Bacteriophage (phage) vB_EcoM_CBA120, discovered by Kutter and colleagues, is a member of the recently defined Kuttervirus genus of contractile tailed phages belonging to the Ackermannviridae family. Each TSP recognizes a different lipopolysaccharide on the membrane of a different bacterial host. The 335 N-terminal residues of TSP4 promote the assembly of the TSP complex and anchor it to the tail baseplate.

However, the SeMet TSP4-N335 containing three constitutive methionines and three additional engineered methionines designed to increase the anomalous signal (Leu12Met, Ile31Met and Leu145Met), were all twinned when grown in KNa-tartrate solution. Thus, phase determination was performed with SeMet protein crystals grown from solutions containing lithium sulfate. The diffraction quality was rather poor and required five merged data sets to yield sufficient anomalous diffraction signal for the identification of 15 Se sites, corresponding to 5 SeMet residues per monomer. Phase determination by the SAD method yielded an electron density map that enabled the building of the AD-XD1-XD2 trimer. However, the electron density associated with the XD3 domains could not be traced. The crystal structure of TSP4-N335 reveals a trimeric protein comprising four domains. The XD2 and XD3 domains share the same threefold symmetry axis as the AD and XD1 domains such that three XD2 domains splay apart and do not interact with one another whereas the three XD3 domains pack together around the threefold symmetry axis. A linker (Gly179-Leu-Gly-Gln-Gly-Arg-Val-Tyr-Ser-Arg188) that connects the XD1 and XD2 domains exhibits a well-defined conformation in the two TSP4-N335 crystal structures. The third linker connects the TSP4 XD2 and XD3 domains by a glycine-rich flexible long polypeptide (Thr250-Pro-Ile-Gln-Leu-Gly-Asn-Gly-Gly-Gly-Ser-Gly-Ser-Ser-Thr264) that is structurally disordered as manifested by the lack of associated interpretable electron density maps for both the wild-type and SeMet TSP4-N335 crystal structures.

>MANKPTQPLFPMGLETSESSNIKGFNNSGTMEHSPGAVMTFPEDTEVTGLPSSVRYNPDSDEFEGYYENGGWLSLGGGGIRWETLPHAPSSNLLEGRGYLINNTTGTSTVVLPSPTRIGDSVTICDAYGKFATYPLTVSPSGNNMYGSTEDMAITTDNVSATFTWSGPEQGWVITSGVGLGQGRVYSREIFTQILASETSAVTLNTPPTIVDVYADGKRLAESKYSLDGNVITFSPSLPASTELQVIEYTPIQLGNGGGSGSSTITWVYNGGSAIGGETEITLDIVVDDVPAIDINGSRQYKNLGFTFDPLTSKITLAQELDAEDEVVVIINGTPHHHHHH[3x]>[4x]SNADADVQPAGSVPIPDGPAQTWIVADLDSGQVLAGRDQNVAHPPASTIKVLLALVALDELDLNSTVVADVADTQAECNCVGVKPGRSYTARQLLDGLLLVSGNDAANTLAHMLGGQDVTVAKMNAKAATLGATSTHATTPSGLDGPGGSGASTAHDLVVIFRAAMANPVFAQITAEPSAMFPSDNGEQLIVNQDELLQRYPGAIGGKTGYT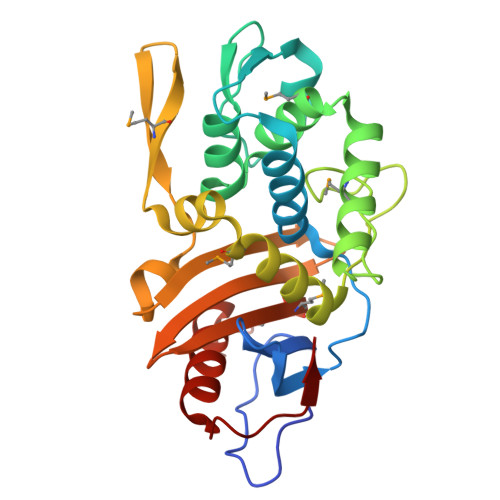NAARKTFVGAAARGGRRLVIAMMYGLVKEGGPTYWDQAATLFDWGFALNPQASVGSL> MAHHHH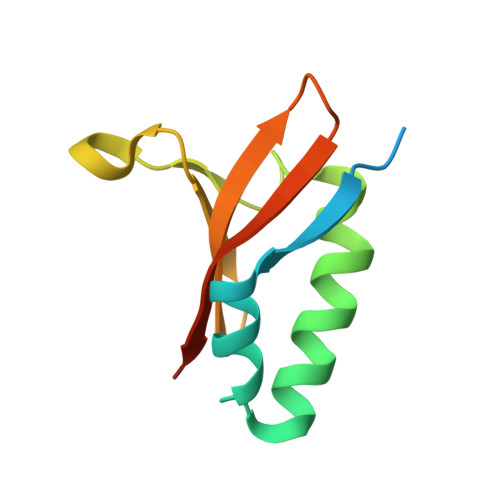HHVDDDDKMVPYTVRFTTTARRDLHKLPPRILAAVVEFAFGDLSREPLRVGKPLRRELAGTFSARRGTYRLLYRIDDEHTTVVILRVDHRADIYRR> MTTSAASQASLPRGRRTARPSGDDRELAILATAENLLEDRPLADISVDDLAKGAGISRPTFYFYFPSKEAVLLTLLDRVVNQADMALQTLAENPADTDRENMWRTGINVFFETFGSHKA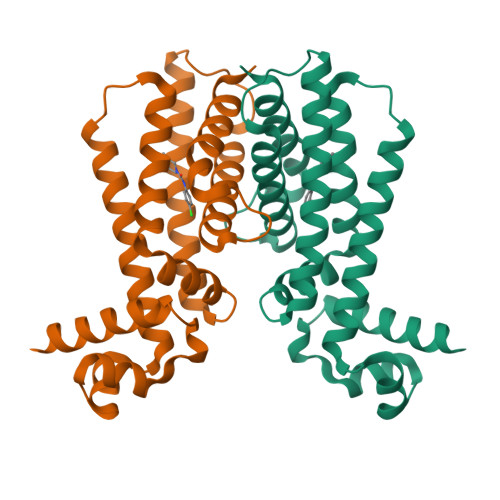VTRAGQAARATSVEVAELWSTFMQKWIAYTAAVIDAERDRGAAPRTLPAHELATALNLMNERTLFASFAGEQPSVPEARVLDTLVHIWVTSIYGENR> XPPGPPGPPGPR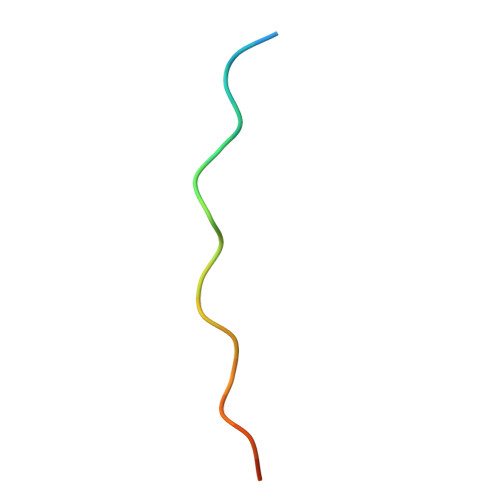GPPGPPGX>GMSETATWQPSASIPNLLKRAAIMAEIRRFFADRGVLEVETPCMSQATVTDIHLFPFETRFVGPGHSQGINLYLMTSPEYHMKRLLAAGCGPVFQLCRSFRNEEMGRHHNPEFTMLEWYRPHYDMYRLMNEVDDLLQ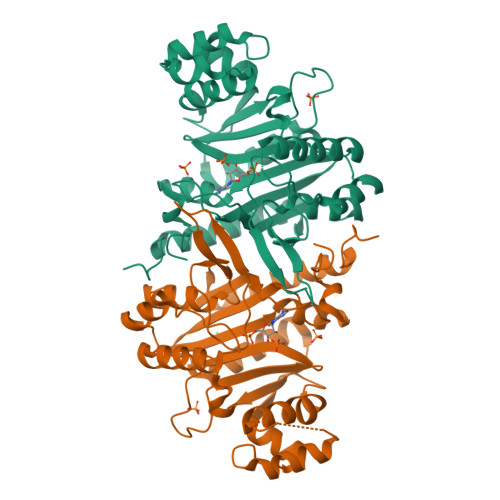QVLDCQPAESLSYQQAFQRHLEIDPLSADKTQLREAAAKLDLSNIADTEEDRDTLLQLLFTMGVEPHIGKEKPTFIYHFPASQASLAQISTEDHRVAERFEVYYKGIELANGFHELTDAREQQQRFEQDNRKRAARGLPQQPIDQNLLDALAAGLPDCSGVALGVDRLVMLALGAESLADVIAFTVDRA[2x]> MAHHHHHHMATPHNSAKVGDFAETVLMCGDPLRAKLIADNYLENAKQVNSVRGMLGFTGTYKGKPLSVMGHGMGIPSISIYAEELYNVYKVKTIIRVGTCGTVDPNVHVRDVCIVTASGTDSNVNRMRLLGHDFPATANFEV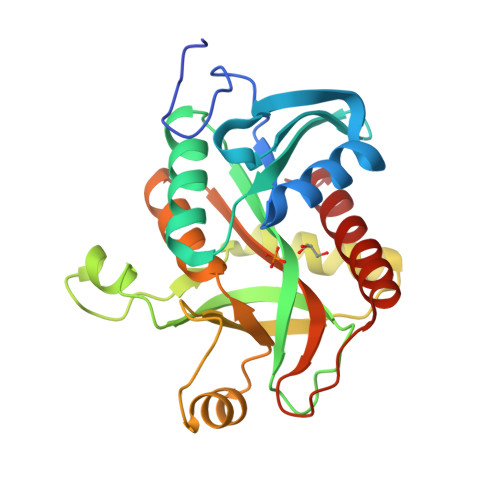VSALVESAKALNIPTQVGKAYSTDIFYSKEQGLNEALAQYHFIAVEMESAGLFPIADYYGARAGCICTVSDHIITHESATPEERQTSFQNMIKIALEATLKL>[4x]MSKPQPIAAANWKCNGSQQSLSELID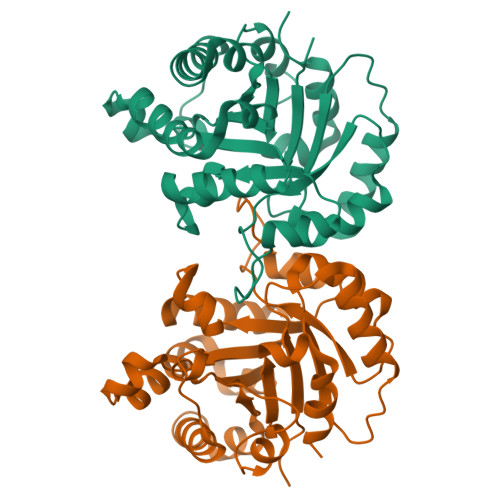LFNSTSINHDVQCVVASTFVHLAMTKERLSHPKFVIAAQNAIAKSGAFTGEVSLPILKDFGVNWIVLGHSERRAYYGETNEIVADKVAAAVASGFMVIACIGETLQERESGRTAVVVLTQIAAIAKKLKKADWAKVVIAYEPVWAAGTGKVATPQQAQEAHALIRSWVSSKIGADVAGELRILYGGSVNGKNARTLYQQRDVNGFLVGGASLKPEFVDIIKATQ>MKFFDGVKDVLSGLINRRNSMARNRVSHRYLSDEEMRVMYKAGLMSKIIRLKAG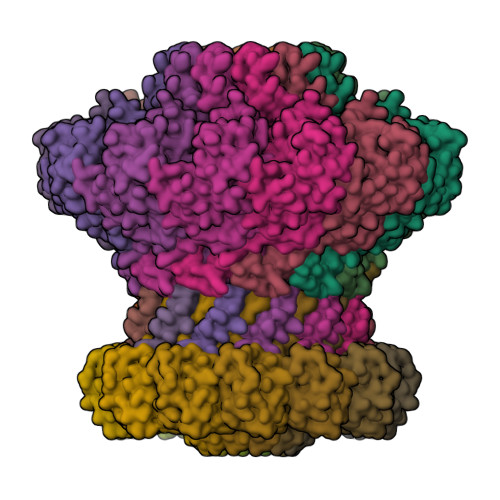YALNDTLKFESTQDQEIYKKRLSKHVKNATKFMLGFGRGVIVVFKNGDDLSKPLERGVDPKLLKIRVFSGDIAKGNNPDNDLRSERYYKPKNYTIKGHTIHWTRVVDFTYYMPSENELPDYYYGGMSESELIYEQFINDSVVQRASGSIIEKASTFVYKIKGYKQLIQAKKEEDIIKYVSTCEDGRSIYGGLITDADDEVSTLTQSLTDLDKVDNVTLRRIAMVTGLGMTVLIGEQASGLNASGEKERQGFQDTIENLQSDYLEDPLNRLAEIFQLGFIEFKDNQGQSANERVEYDKKAVDVAKVLWELGEDYGAYLKDKDVVQADDWDNFWKEKDENSEVDESLPLGDLFSSGDVNG[12x];>MALIDDFKARFPNLDGSLVDALVPVYENNYSCYYGGSYENDCDKEAILLLIAHLVVTDPSYSGDESSSRAVASQSVGSVSVSFVAGSTGSDWTNWLNSTRYGQLFLMVTSNNMGPSFA[12x]>GAGAGAGAGAGMFRLTRLSNKPILSPIKEHEWEKEAVFNAAVIYEGNKFHLFYRASNNKFVLNTEKPEEKYKFVSSIGYAVSEDGINFERFDKPVLVGEIPQEAWG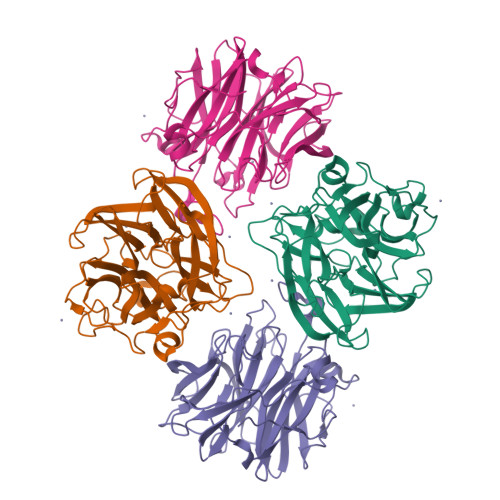VEDPRITKIDNKYYMLYTGFGGRDWLDFRICMVWSDDLKNWKGHRIVLDEPNKDAALLSEKINGKYVLFHRRMPDIWIAYSDDLVNWYNHKIIMSPKSHTWESKKIGIAGPPIKREDGWLLIYHGVDNNNVYRLGVALLDLKDPSKVIARQKEPILEPELDWEINGLVPNVVFSCGAVEVNDMYYVYYGAADTHIGVAVIEKEKVKF[4x]>[2x]MEDSLYSLLVAELAGQRNRFDIALSNYVVQAQKTRDPGVSERAFRIAEYLGADQEALDTSLLWARSAPDNLDAQRAAAIQLARAGRYEESMVYMEKVLNGQGDTHFDFLALSAAETDPDTRAGLLQSFDHLLKKYPNNGQLLFGKALLLQQDGRPDEALTLLEDNSASRHEVAPLLLRSRLLQSMKRSDEALPLLKAGIKEHPDDKRVRLAYARLLVEQNRLDDAKAEFAGLVQQFPDDDDLRFSLALVCLEAQAWDEARIYLEELVERDSHVDAAHFNLGRLAEEQKDTARALDEYAQVGPGNDFLPAQLRQTDVLLKAGRVDEAAQRLDKAR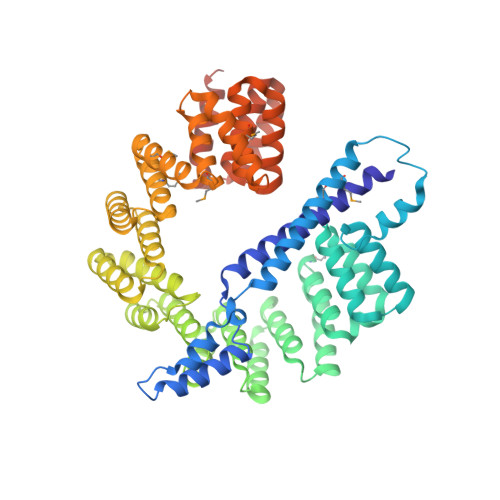SEQPDYAIQLYLIEAEALSNNDQQEKAWQAIQEGLKQYPEDLNLLYTRSMLAEKRNDLAQMEKDLRFVIAREPDNAMALNALGYTLADRTTRYGEARELILKAHKLNPDDPAILDSMGWINYRQGKLADAERYLRQALQRYPDHEVAAHLGEVLWAQGRQGDARAIWREYLDKQPDSDVLRRTIKRLTGAETPKLAAALEHHHHHH>[2x]AEEKAKAVPLIHQEGNRLYREGHVKEAAAKYYDAIACLKNLQMKEQPGSPEWIQLDQ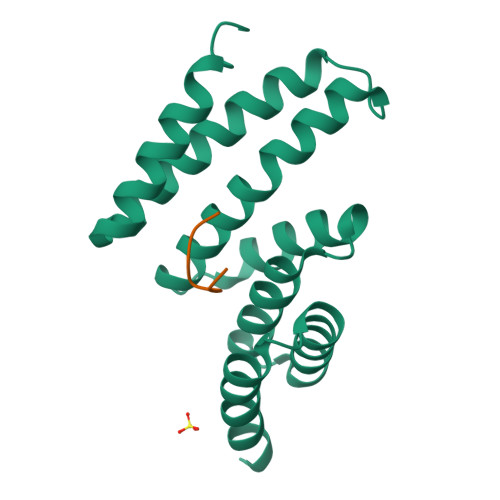QITPLLLNYCQCKLVVEEYYEVLDHCSSILNKYDDNVKAYFKRGKAHAAVWNAQEAQADFAKVLELDPALAPVVSRELQALEARIRQ;>[2x]SRMEEVD>[8x]G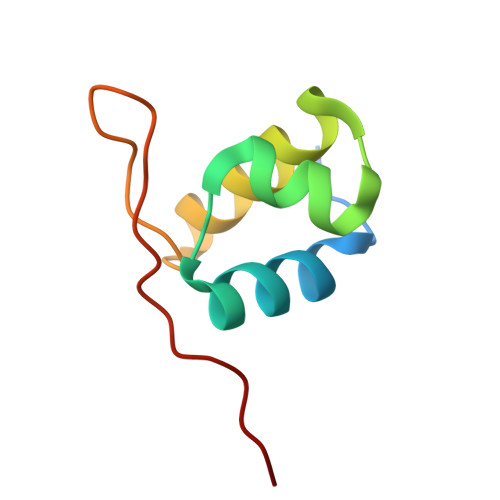SGEGSEDDPLYDEAVRFVTESRRASISAVQRKLKIGYNRAARMIEAMEMAGVVTPMNTNGSREVIAPAPVRD>[2x]ACTKNAIAQTGFNKDKYFNGDVWYVTDYLNLQPDNVPKRYCAALAAGTASGKLKEALYHYDPKTQDTFYDVSELQVE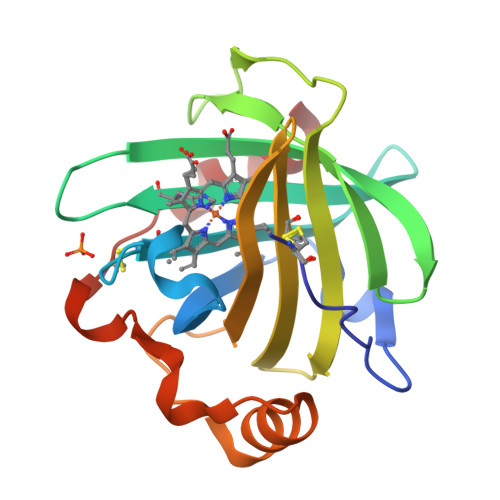SLGKYTANFKKVDKNGNVKVAVTAGNYYTFTVMYADDSSALIHTCLHKGNKDLGDLYAVLNRNKDAAAGDKVKSAVSAATLEFSKFISTKENNCAYDNDSLKSLLTK>GHKEFDYFTLALTWSGTECLSVKDSCPTNACSRSEVETGFTIKGLWPDYDDGTWPSCCEGAKYDQNEISILSNDLSKYWPSYSCPSSSACGSFDASDLAY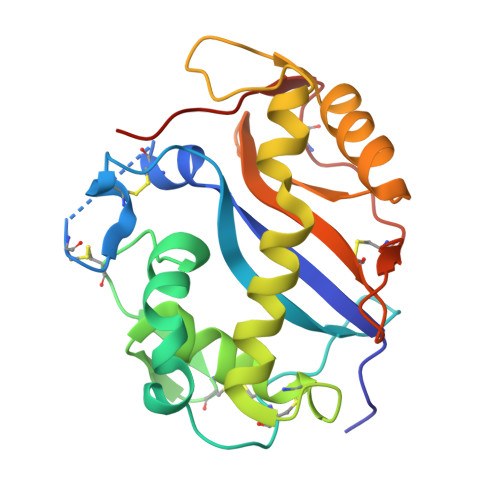EWAKHGTCSSPVLGNQYEYFSTTLMLYFKYNISEILSESGYLPSNTAEYKVEGIMSAIQSALRVTPVVKCKSDAVEQVQICFDKTLQLQECPSTASTCPSLVSLPIKNTIKP[2x]>TPRGFVVHTAPVGLADDGRDDFTVLASTAPATVSAVFTRSRFAGPSVVLCREAVADGQARGVVVLARNANVATGLEGEENAREVREAVARALGLPEGEMLIASTGVIGRQYPMESIREHLKTLEWPAGEGGFDRAARAIMTTDTRPKEVRVSVGGATLVGIAKGVGMLEPDMA[4x];>[4x]ALLTFFATDARLDPAEQDRLFRRVMDRTFNAVSIDTDTSTSDTAVLFANGLAGEVDAGEFEEALHTAALALVKDIASDGEGAAKLIEVQVTGARDDAQAKRVGKTVVNSPLVKTAVHGCDPNWGRVAMAIGKCSDDTDIDQERVTIRFGEVEVYPPKARGDQADDALRAAVAEHLRGDEVVIGIDLAIADGAFTVYGCDLTEGYVRL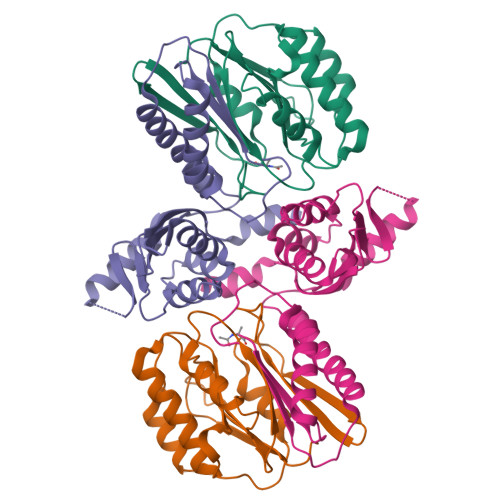NSEYTT> MDEASHLPNGSLKNMEFTPVGFIKSKRNTTQTQVVSPTKVPNANNGDENEGPVKKRQRRSIDDTIDSTRLFSEASQFDDSFPEIKANIPPSPRSGNVDKSRKRNLIDDLKKDVPMSQPLKEQEVREHQMKKERFDRALESKLLGKRHITYANSDISNKELYINEIKSLKHEIKELRKEKNDTLNNYD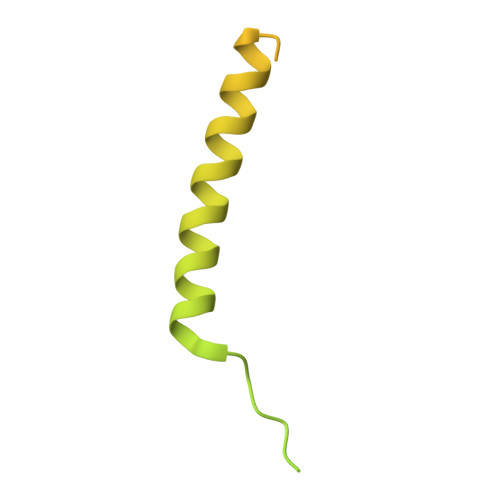TLEEETDDLKNRLQALEKELDAKNKIVNSRKVD> MKIAIINMGNNVINFKTVPSSETIYLFKVISEMGLNVDIISLKNGVYTKSFDEVDVNDYDRLIVVNSSINFFGGKPNLAILSAQKFMAKYKSKIYYLFTDIRLPFSQSWPNVKNRPWAYLYTEEELLIKSPIKVISQGINLDIAKAAHKKVDNVIEFEYFPIEQYKIH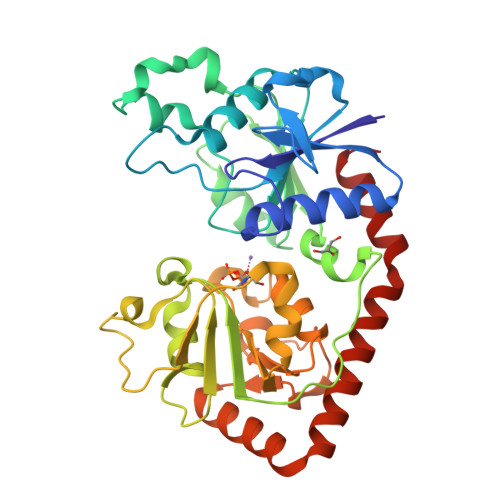MNDFQLSKPTKKTLDVIYGGSFRSGQRESKMVEFLFDTGLNIEFFGNAREKQFKNPKYPWTKAPVFTGKIPMNMVSEKNSQAIAALIIGDKNYNDNFITLRVWETMASDAVMLIDEEFDTKHRIINDARFYVNNRAELIDRVNELKHSDVLRKEMLSIQHDILNKTRAKKAEWQDAFKKAIDL[(3~{R})-3-carboxy-7-[(4-methylnaphthalen-1-yl)methyl]-5-oxidanylidene-2,3-dihydro-[1,3]thiazolo[3,2-a]pyridin-8-yl]-dimethyl-azanium 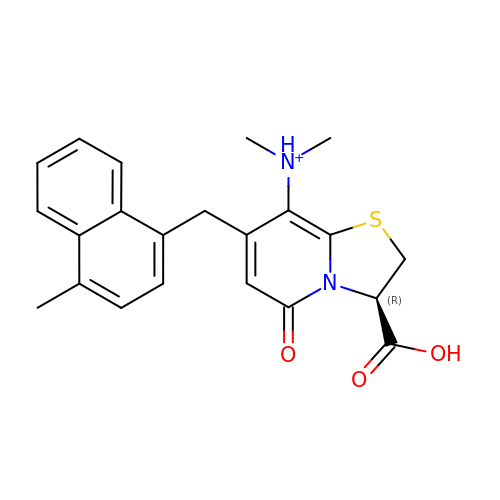| C22 H23 N2 O3 S | JKRFTQGEDGJQEE-SFHVURJKSA-O> GUUAAUCAUGCUCGGGUAAUCGCUGCGGCCGGUUUCGG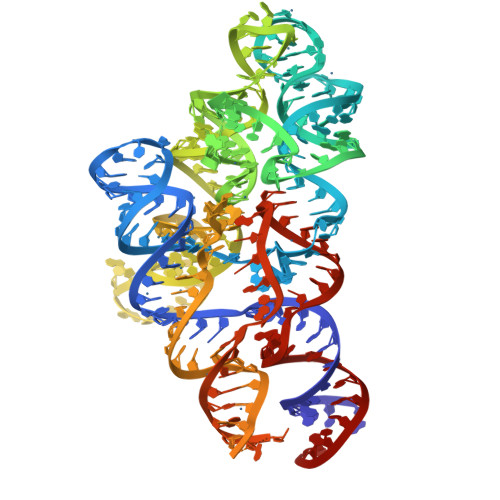CCGUAGAGGAAAGUCCAUGCUCGCACGGUGCUGAGAUGCCCGUAGUGUUCGUGGAAACACGAGCGAGAAACCCAAAUGAUGGUAGGGGCACCUUCCCGAAGGAAAUGAACGGAGGGAAGGACAGGCGGCGCAUGCAGCCUGUAGAUAGAUGAUUACCGCCGGAGUACGAGGCGCAAAGCCGCUUGCAGUACGAAGGUACAGAACAUGGCUUAUAGAGCAUGAUUAACGUC>MGAMIVKEVYETAEKIKSMEI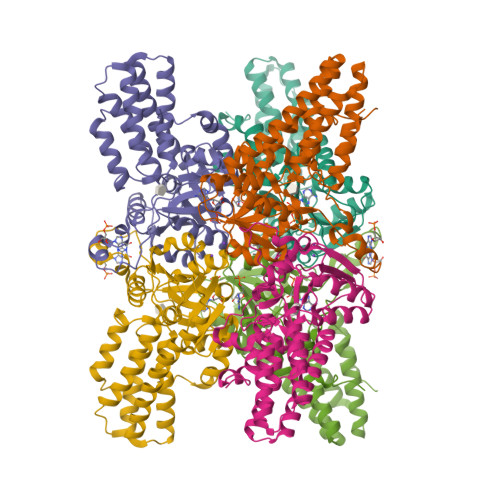RGAGRIARAAAQALMIQAEKSKAKEPEELWNELKVASKILYNTRPTAVSLPNALRYVMHRVKAAYLGGADLETLRFTAINSAKEFIYNSEKAIERIGEIGAKRIEDGDIIMTHCHSKAAISVMKKAFEQGKNIKVIVTETRPKWQGKITAKELASYGIPVIYIVDSAARHYMKMTDKVVMGANSITANGAVINKIGTSLIALTAKEHRVWVMIAAETYKFHPATMLGQLVEIEMRDPTEVIPEEELRTWPKNIEVWNPAFDVTPPEYIDVIITERGIIPPYAAIDILKEEFGWALKYKEPWED[3x]>[2x]GMTTWKEL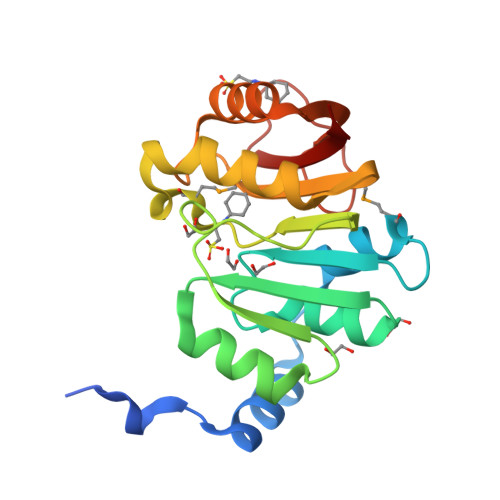TDNNPAHSENYAQRWRNLAAAGNDIYGEARLIDAMAPRGAKILDAGCGQGRIGGYLSKQGHDVLGTDLDPILIDYAKQDFPEARWVVGDLSVDQISETDFDLIVSAGNVMGFLAEDGREPALANIHRALGADGRAVIGFGAGRGWVFGDFLEVAERVGLELENAFESWDLKPFVQGSEFLVAVFTKK> SESSIENFLCRSACVYMGEYHTTNTDTSKLFASWTINAR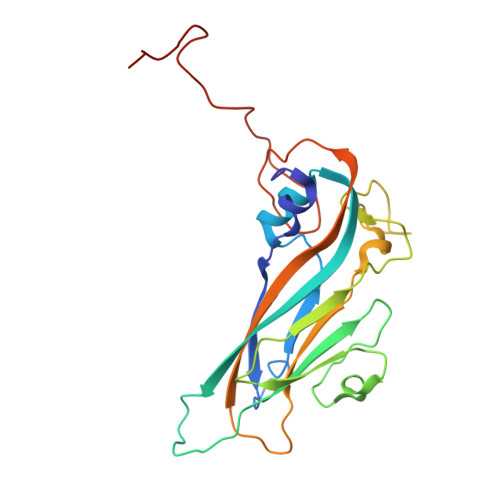RMVQMRRKLELFTYVRFDMEVTFVITSKQDQGTQLGQDMPPLTHQIMYIPPGGPIPKSVTDYTWQTSTNPSIFWTEGNAPPRMSIPFISIGNAYSNFYDGWSHFSQNGVYGYNTLNHMGQIYVRHVNGSSPLPMTSTVRMYFKPKHVKVWVPRPPRLCQYKNASTVNFTPTNITEKRQSINYIPETV> DTDFVPPSP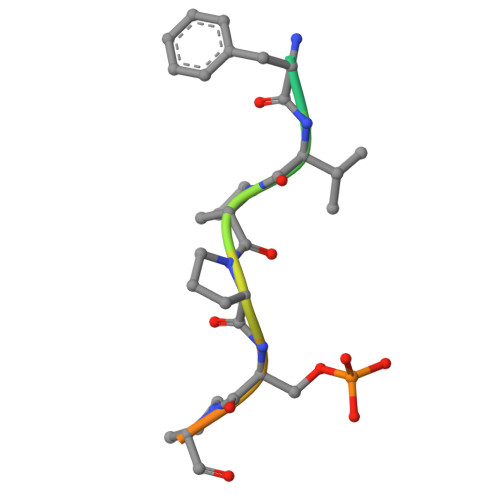EEII>[2x]MEALVLVGHGSRLPYSKELLVKLAEKVKERNLFPIVE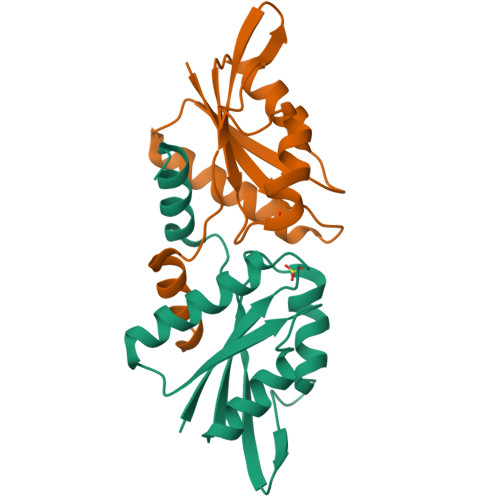IGLMEFSEPTIPQAVKKAIEQGAKRIIVVPVFLAHGIHTTRDIPRLLGLDENGCGTLEIDGKTVEIIYREPIGADDRIVDIIIDRAFGR>MDPVYVDIDADSAFLKALQRAYPMFEVEPRQVTPNDHANARAFSHLAIKLIEQEIDPDSTILDIGSAPARRMMSDRKYHCVCPMRSAEDPERLANYARKLASAAGKVLDRNISGKIGDLQAVMAVPDTETPTFCLHTDVSCRQRADVAIYQDVYAVHAPTSLYHQAIKGVRLAYWVGFDTTPFMYNAMAGAYPSYSTNWADEQVLKAKNIGLCSTDLTEGRRGKLSIMRGKKLEPCDRVLFSVGSTLYPESRKLLKSWHLPSVFHLKGKLSFTCRCDTVVSCEGYVVKRITMSPGLYGKTTGYAVTHHADGFLMCKTTDTVDGERVSFSVCTYVPATICDQMTGILATEVTPEDAQKLLVGLNQRIVVNGRTQRNTNTMKNYMIPVVAQAFSKWAKECRKDMEDEKLLGVRERTLTCCCLWAFKKQKTHTVYKRPDTQSIQKVQAEFDSFVVPSLWSSGLSIPLRTRIKWLLSKVPKTDLTPYSGDAQEARDAEKEAEEEREAELTLEALPPLQAAQEDVQVEIDVEQLEDRAGA[24x]

NsP1 is the membrane anchor for the complex, forming dodecameric pores that associate monotopically with the membrane in the necks of the spherules to gate their entrance. Enzymatically, nsP1 also has a role in addition of cap0 structures to the 5′ end of the positive-sense viral RNAs. NsP1 possesses both N′7 methyltransferase and guanylyltransferase activity and reverses the order of these reactions. Each nsP1 protomer is built around a methyltransferase fold common to SAM-dependent methyltransferases with additional insertions (membrane binding and oligomerisation (MBO) loops 1 and 2) and extensions (ring aperture membrane binding oligomerisation (RAMBO) domain) that contribute to pore formation, oligomerization, and membrane binding.

To better understand the initiating methylation step of GTP in the nsP1 pathway, we solved the cryo-EM structures of detergent solubilized nsP1 pores in the presence of a 100-fold molar excess of SAM or GTP substrates. Common to other N7-SAM dependent methyltransferases (N7 MTases), the SAM ligand binds in a pocket near the switch point of the Rossmann fold in the capping domain. The density for the SAM ligand is not fully defined in the binding pocket, where in maps reconstructed with symmetry, only density for the base and ribose moieties is clearly visible. In comparison with the apo form of nsP1, neighboring helices αB and C are very poorly defined and overall local resolution for this region is worse compared to the apo and other bound states. Contacts made to the SAM ligand are primarily weak van der Waal’s (VdW) interactions, involving residues I64-A67 from the DIG motif and P83, R85, T137 and D138 to the base; S86, D89, and R92 from the DPER motif to the ribose and residues R70, G151, and D152 to the methionine. The SAM base forms a hydrogen bond (H-bond) between N6 and the side chain of residue T137 in nsP1, which maintains a second H-bond with R85. The purine base is bound in the anti-conformation to the ribose, where the 2′ and 3′ hydroxyl groups of the ribose form H-bonds to the side chains of D89 of helix αB. Although the density for the methionine is quite poorly resolved, its position replaces the side chain of R70 in the apo form of nsP1, which is also poorly defined in the structure. Taken all together, these data suggest that in the absence of GTP, SAM is not stably bound, and does not satisfy some of the contacts required for correct positioning of the substrate for methyl transfer. The correlation between the presence of SAM in the active site and the disordering of helixes αC and αB suggests that binding of the SAM alone also induces significant destabilization of part of the nsP1 capping domain.> HGFVSGIVADGSYYGGYNTDEYPYMSNP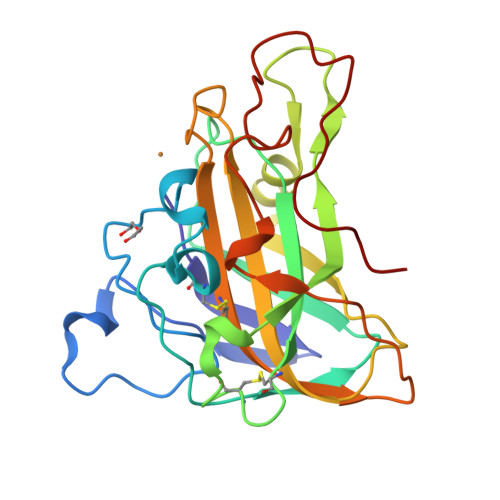PNVIAWSTTATNCGFTNGTGYQSPDIICHSNASNGSNTAVVAAGSSIQFQWTVWPASHHGPLITYLAPCGGNCATVDKTTLDFTKIAAVGLVNGVSPPGVWADDSMIADNNTAVVVIPASYAPGNYVLRHEIIALHVAGNNNGAQNYPQCFNIQITGGGSAQGSGVAGTSLYKNTDPGIKFNIYSDLSGGYPIPGPALFA>DPGLNSKIAQLVSMGFDP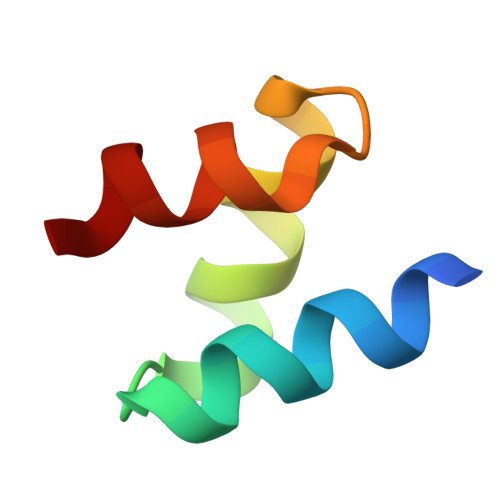LEAAQALDAANGDLDVAASFLL[2x]>[2x]MIDLAIGQVPIANWVSSATDWITSTFSSGFDVIQKSGTVLMNGITGALTAVPFWLMIAVVTILAILVSGKKIAFPLFTFIGLSLIANQGLWSDLMSTITLVLLSSLLSIIIGVPLGIWMAKSDLVAKIVQPILDFMQTMPGFVYLIPAVAFFGIGVVPGVFASVIFALPPTVRMTNLGIRQVSTELVEAADSFGSTARQKLFKLEFPLAKGTIMAGVNQTIMLALSMVVIASMIGAPGLGRGVLAAVQSADIGKGFVSGISLVILAIIIDRFTQKLNVSPLEKQGNPTVKKWKRGIALVSLLALIIGAFSGMSFGKTASDKKVDLVYMNWDSEVASINVLTQAMKEHGFDVKTTALDNAVAWQTVANGQADGMVSAWLPNTHKTQWQKYGKSVDLLGPNLKGAKVGFVVPSYMNVNSIEDLTNQANKTITGIEPGAGVMAASEKTLNSYDNLKDWKLVPSSSGAMTVALGEAIKQHKDIVITGWSPHWMFNKYDLKYLADPKGT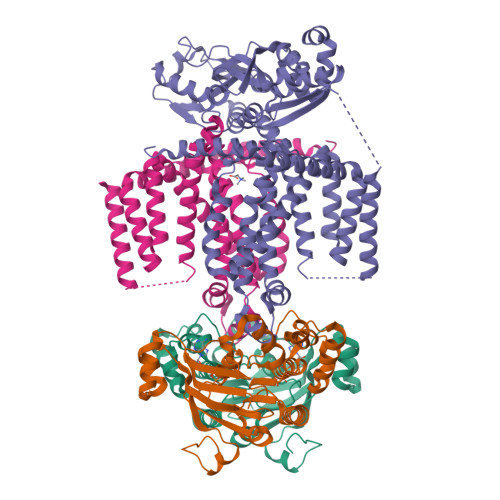MGTSENINTIVRKGLKKENPEAYKVLDKFNWTTKDMEAVMLDIQNGKTPEEAAKNWIKDHQKEVDKWFKGSIEGRHHHHHH;>[2x]MAVKIKIEHLTKIFGKRIKTALTMVEKGEPKNEILKKTGATVGVYDTNFEINEGEIFVIMGLSGSGKSTLLRLLNRLIEPTSGKIFIDNQDVATLNKEDLLQVRRKTMSMVFQNFGLFPHRTILENTEYGLEVQNVPKEERRKRAEKALDNANLLDFKDQYPKQLSGGMQQRVGLARALANDPEILLMDQAFSALDPLIRREMQDELLELQAKFQKTIIFVSHDLNEALRIGDRIAIMKDGKIMQIGTGEEILTNPANDYVKTFVEDVDRAKVITAENIMIPALTTNIDVDGPSVALKKMKTEEVSSLMAVDKKRQFRGVVTSEQAIAARKNNQPLKDVMTTDVGTVSKEMLVRDILPIIYDAPTPLAVVDDNGFLKGVLIRGSVLEALADIPDEDEVEEIEKEEENK> GGGRPTEIENINPNVYDRIKERVLTANEEDENVPDPFDKREIFDLIRNINDPEHPLTLEELHVVQEDLIRINDSQNSVHISFTPTIPHCSMATLIGLSIRVKLLRSLPPRFKVTVEITPGTHASELAVNKQLADKERVAAALENNHLAEVINQCIAAKG;> GGGRGRLILEHTLQGHKGRIWGVAWHPKGNVFASCGEDKAIRIWSLTGNTWSTKTILSDGHKRTIREIRWSPCGQYLASASFDATTAIWSKSSGEFECNATLEGHENEVKSVSWSRSGGLLATCSRDKSVWIWEVAGDDEFECAAVLNPHTQDVKRVVWHPTKDILASASYDNTIKMF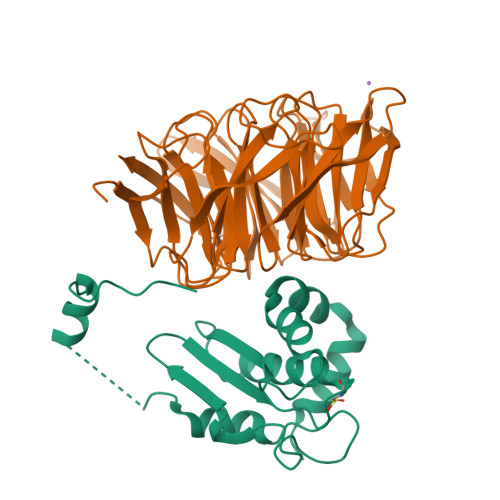AEEPIDNDWDCTATLTSHTSTVWGIDFDADGERLVSCSDDTTIKIWRAYHPGNTAGVATPDQQTVWKCVCTVSGQHSRAIYDVSWCKLTGLIATACGDDGIRIFKESSDSKPDEPTFEQITAEEGAHDQDVNSVQWNPVVAGQLISCSDDGTIKIWKVTE>[2x]MH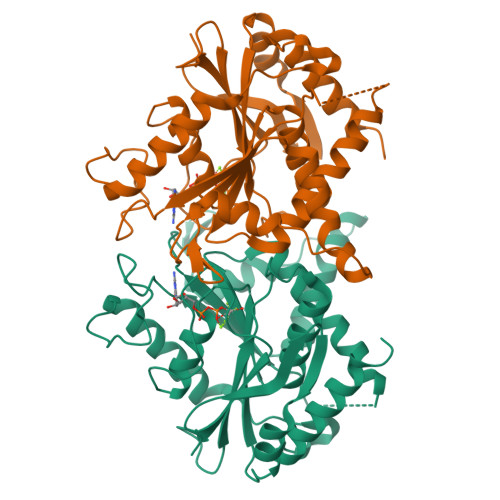HHHHHMRGSMASEIHMTGPMCLIENTNGRLMANPEALKILSAITQPMVVVAIVGLYRTGKSYLMNKLAGKKKGFSLGSTVQSHTKGIWMWCVPHPKKPGHILVLLDTEGLGDVEKGDNQNDSWIFALAVLLSSTFVYNSIGTINQQAMDQLYYVTELTHRIRSKSSPDENENEVEDSADFVSFFPDFVWTLRDFSLDLEADGQPLTPDEYLTYSLKLKKGTSQKDETFNLPRLCIRKFFPKKKCFVFDRPVHRRKLAQLEKLQDEELDPEFVQQVADFCSYIFSNSKTKTLSGGIQVNGPRLESLVLTYVNAISSGDLPCMENAVL>VETISFSFSEFEPGNNDLTLQGAAIITQSGVLQLTKINQNGMPAWDSTGRTLYTKPVHIWDMTTGTVASFETRFSFSIEQPYTRPLPADGLVFFMGPTKSKPAQGYGYLGVFNNSKQDNSYQTLAVEFDTF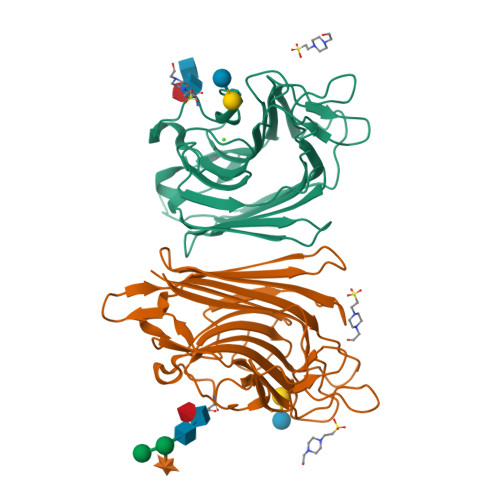SNPWDPPQVPHIGIDVNSIRSIKTQPFQLDNGQVANVVIKYDASSKILLAVLVYPSSGAIYTIAEIVDVKQVLPEWVDVGLSGATGAQRDAAETHDVYSWSFHASLPETND[2x]>[2x]MSQLVLILGDQLSPSIAALDGVDKKQDTIVLCEVMAEASYVGHHKKKIAFWFSAMRHFAEELRGEGYRVRYTRIDDADNAGSFTGEVKRAIDDLTPSRICVTEPGEWRVRSEMDGFAGAFGIQVDIRSDRRFLSSHGEFRNWAAGRKSLTMEYFYREMRRKTGLLMNGEQPVGGRWNFDAENRQPARPDLLRPKHPVFAPDKITKEVIDTVERLFPDNFGKLENFGFAVTRTDAERALSAFIDDFLCNFGATQDAMLQDDPNLNHSLLSFYINCGLLDALDVCKAAERAYHEGGAPLNAVEGFIRQIIGWREYMRGIYWLAG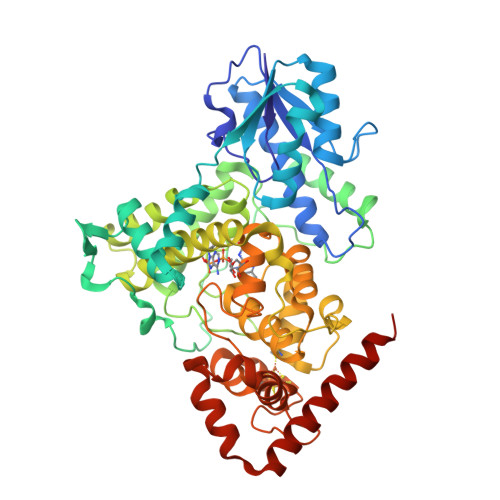PDYVDSNFFENDRSLPVFYWTGKTHMNCMAKVITETIENAYAHHIQRLMITGNFALLAGIDPKAVHRWYLEVYADAYEWVELPNVIGMSQFADGGFLGTKPYAASGNYINRMSDYCDTCRYDPKERLGDNACPFNALYWDFLARNREKLKSNHRLAQPYATWARMSEDVRHDLRAKAAAFLRKLDAAALEHHHHHH> QGPTSIWTKGVTPPTNFIEGTDGSHAPYIANQGWYDITKTFNGKDDLLSAAATAGNMLHWWFDQNKNQIEGYLTEHPEKQAIIFNGEQMFDVKEAISTKDRQLDSKLFEYFKEKAFPTLSARRRGVFPDHVIDMFINGYRLSLDNYDKTPVKEGNKDLRGGIFDQVFTRGDQSKLLTNRYNLRTKTINEISQLIKQELIAGKALAISHTYNNIGISHVINLWGADFNSEGNLEAIYVTDSDSNASIGMKKYYVGVNSAGEV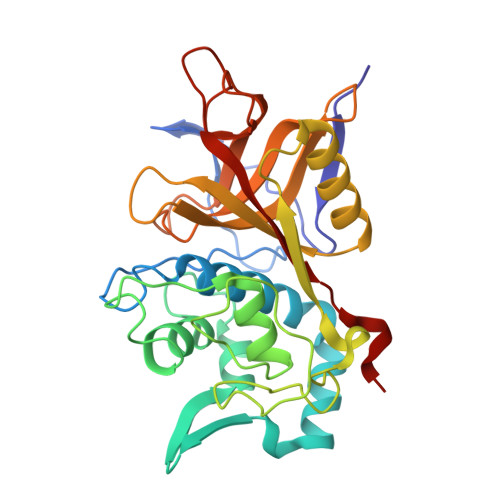AVSSKKIDSEHLGAAALGLYTLSAGQGIWH>MSLEGKTIGITAIGTDHDWDLKAYQAQIAEIERLGGTAIALDAGRNDQTQVSQIQTLIAQKPDAIIEQLGNLDVLNPWLQKINDAGIPLFTVDTATPHAINNTTSNNYSIGAELALQMVADLGGKGNVLVFNGFYSVPVCKIRYDQMKYVLEAFPDVKIIE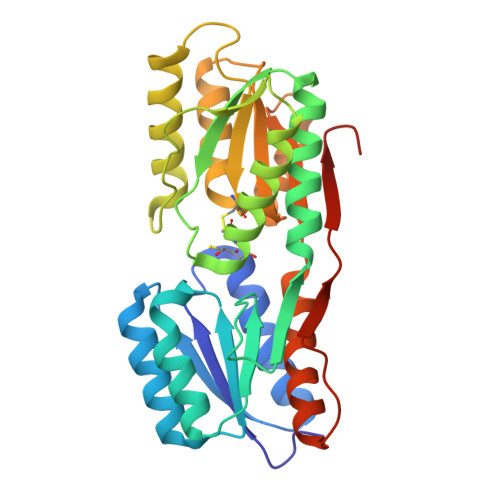PELRDVIPNTIQSAYSNVTDMLTKYPNEGDVGAIWACWDVPMIGATQALQAAGRTDIRTYGVDGSPEFVEMVADPESPAGAVAAQQPSEIGKLAVQNVARHLAGQEVKPFTFAPAVLITKENEGHHHHHH[4x]> SNAERALLQLVVEDDAKALVFVLGQDARRYFEEELPASPFEFPSPQAVANSRQNVGVMFLDKLQYLYMYLTKLEVDEAPEYRTLVVYGLEQLLGAGGELDA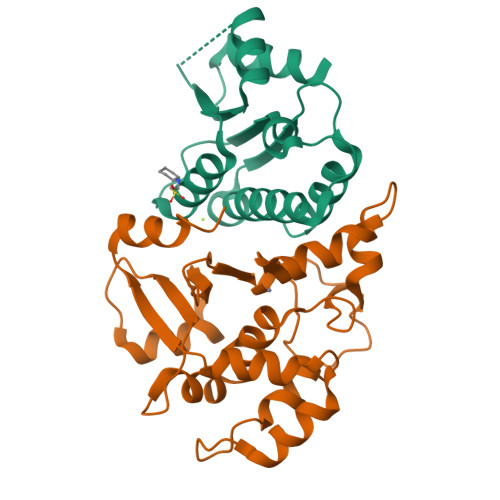DQVRLASLIYNTAFRVRVRHGAAVRFVAHGAPHAQLQQLEAHWRLFT;> MAETNFNYSKLLRNLVTEDNVLNEVVVSFLYQLFPRDLFVRAFSLLESADMFIYVWMPTPKEADELLESLYNGTPLYRPIVRPRGPDDRPVCVDLDHWFCSCTEFAATCRPHLVGDTPLSDALFRPTEAADPDDCFGMLAGLQHLRADPEKLMCEHLFAFAILLQTDLRVLRHFSTGPGAQVFVLGITSIDEWLKLHLNVV>[2x]GPSSTGVGVIHPFLHQNTSDFMEQRFSSMFTGQEFFLSDHVIKGQRVLPSAAYLEMARAAIQQATGGLDSERELEGLRFKNVVWTQPLAVGPEPVQAHIELYPEANGEIVFEIYSDSKQDRDQTTEIVHSQGSAVLCSIPDIPSFDLSVLQEQCSLRTLSAEQCYDAFKKMGV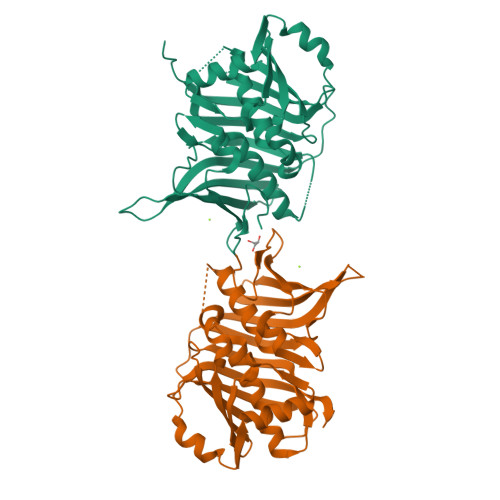DYGPAHRGIEQILIGQEQVLAKLSLPSSVVKTQGQFGLHPSLLDAALQSSLGLMMATSDFSLILPFALEEMVIVGDCSSSMWALIRYREGSKAGDRVEKFDIDLCDENGNVQVRMKGFSTRKIANVSVRSA>METWVLGRRDVAEVVAAVGRDELMRRIIDRLTGGLAEIGRGERHLSPLRGGLERSEPVPGIWEWMPHREPGDHI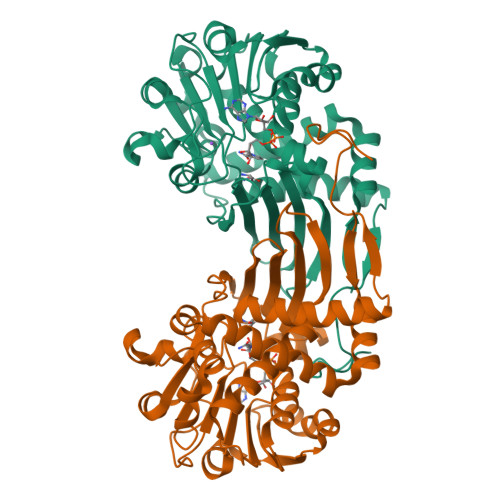TLKTVGYSPANPARFGLPTILGTVARYDDTTGALTALMDGVLLTALRTGAASAVASRLLARPDSHTLGLIGTGAQAVTQLHALSLVLPLQRALVWDTDPAHRESFARRAAFTGVSVEIAEPARIAAEADVISTATSVAVGQGPVLPDTGVREHLHINAVGADLVGKTELPLGLLERAFVTADHPEQALREGECQQLSADRLGPQLAHLCADPAAAAGRQDTLSVFDSTGFAFEDALAMEVFLEAAAERDLGIRVGIEHHPGDALDPYALQ[4x]>[4x]EQVFHFYWLDAYEDQYNQPGVVFLFGKVWIESAETHVSCCVMVKNIERTLYFLPREMKIDLNTGKETGTPISMKDVYEEFDEKIATKYKIMKFKSKPVEKNYAFEIPDVPEKSEYLEVKYSAEMPQLPQDLKGETFSHVFGTNTSSLELFLMNRKIKGPCWLEVKSPQLLNQPVSWCKVEAMALKPDLVNVIKDVSPPPLVVMAFSMKTMQNAKNHQNEIIAMAALVHHSFALDKAAPKPPFQSHFCVVSKPKDCIFPYAFKEVIEKKNVKVEVAATERTLLGFFLAKVHKIDPDIIVGHNIYGFELEVLLQRINVCKAPHWSKIGRLKRSNMPKLGGRSGFGERNATCGRMICDVEISAKELIRCKSYHLSELVQQILKTERVVIPMENIQNMYSESSQLLYLLEHTWKDAKFILQIMCELNVLPLALQITNIAGNIMSRTLMGGRSERNEFLLLHAFYENNYIVPDKQIFRKPQQKLGDE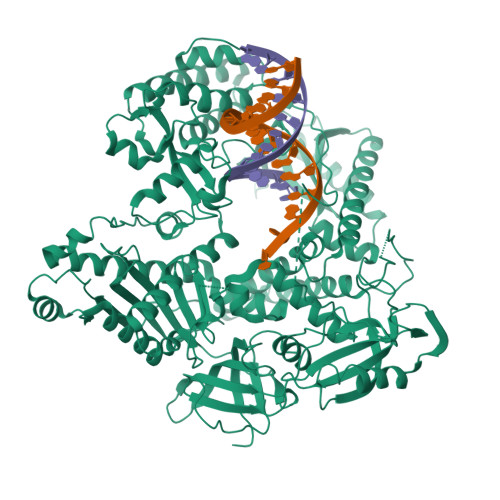DEEIDGDTNKYKKGRKKAAYAGGLVLDPKVGFYDKFILLLDFNSLYPSIIQEFNICFTTVQRVASEAQKVTEDGEQEQIPELPDPSLEMGILPREIRKLVERRKQVKQLMKQQDLNPDLILQYDIRQKALKLTANSMYGCLGFSYSRFYAKPLAALVTYKGREILMHTKEMVQKMNLEVIYGDTDSIMINTNSTNLEEVFKLGNKVKSEVNKLYKLLEIDIDGVFKSLLLLKKKKYAALVVEPTSDGNYVTKQELKGLDIVRRDWCDLAKDTGNFVIGQILSDQSRDTIVENIQKRLIEIGENVLNGSVPVSQFEINKALTKDPQDYPDKKSLPHVHVALWINSQGGRKVKAGDTVSYVICQDGSNLTASQRAYAPEQLQKQDNLTIDTQYYLAQQIHPVVARICEPIDGIDAVLIATWLGLDPTQFRVHHYHKDE ETHYL 4-(3-HYDROXYPHENYL)-6-METHYL-2-THIOXO-1,2,3,4-TETRAHYDROPYRIMIDINE-5-CARBOXYLATE 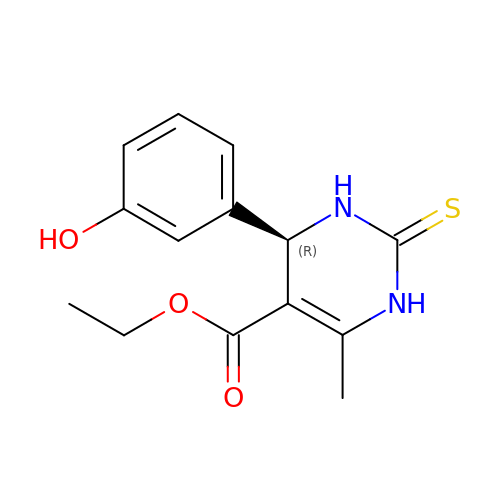| C14 H16 N2 O3 S | LOBCDGHHHHGHFA-LBPRGKRZSA-N> MGTFTLHQGQTNLIKSFFRNYYLNAELELPKDMELREFALQPFGSDTYVRHLSFSSSEELRDYLVNRNLPLHLFYSSARYQLPSARNMEEKAWMGSDLLFDIDADHLCKLRSIRFCPVCGNAVVSEKCERDNVETLEYVEMTSECIKRGLEQTRNLVEILEDDFGLKPKVYFSGNRGFHVQVDCYGNCALLDSDERKEIAEYVMGIGVPGYPGGSENAPGWVGRKNRGINGVTIDEQVTIDVKRLIRIPNSLHGKSGLIVKRVPNLDDFEFNETLS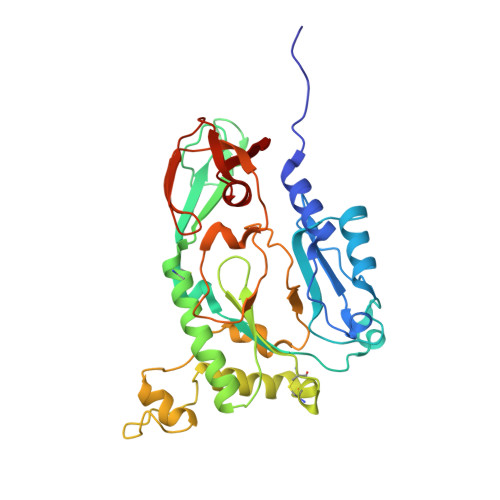PFTGYTIFLPYITIETEVLGSIIKLNRGIPIKIKSSIGIYLHLRNLGEVKAYVR>METILKMGLQANVGSVEYDSAKILSDKISELSDGEMKLLLYPGAQLGDDRAMLQQLSMGDLDITFAEFGRMGLWIPRAEAVMLPYVVKNYAHIQRIFNSKFGQGVREEMLTNFNWRALDTWYNGTRQTSSNRPLNTISDFEGLKLRVPNAKANLAFAKYAGASPTPMVFSEVYLALQTNAVDGQENPLPTFNTMKFYEVQPNLAMTNHIVNDQMVLISEDRWQSLSKDQQATITEAVSVAGKRHTNFVNNQEKELITFFKAEGVNITYPDLAPFREAMLPIYKDFDKKIGKQLVEELSDI[2x]

Tripartite ATP-independent periplasmic (TRAP) transporters are a major class of secondary transporters found in bacteria and archaea—but, not in eukaryotes. First reported over 25 years ago6, they use energetically favourable cation gradients to drive the import of specific carboxylate- and sulfonate-containing nutrients against their concentration-gradient, including C4-dicarboxylates, α-keto acids, aromatic substrates and amino acids. A functional TRAP system is made up of a soluble substrate-binding ‘P-subunit’, and a membrane-bound complex comprising a small ‘Q-subunit’ and a large ‘M-subunit’. The best characterised TRAP transporters are those for sialic acid, otherwise known as the SiaPQM system.

We determined the crystal structure of SiaP bound to Neu5Ac in a closed state at 1.04 Å resolution, as a crystal structure of substrate-loaded SiaP enables us to model the SiaPQM complex. We confirmed that SiaP binds sialic acid with nanomolar affinity and that the crystal structure is representative of the protein structure in solution. The docked structure shows two calliper-like helices of SiaP, α2 at the N-terminal lobe and α5 at the C-terminal lobe of SiaP, interact with the scaffold portion of the M-subunit. Residues R49 and N148 (SiaP) form a latch between the lobes of SiaP at the surface of the substrate binding cleft, enclosing a number of ordered solvent molecules that extend toward the substrate. One hotspot involves the invariant D181 of SiaP immediately prior to β8 and K232 on the loop between TM7 and TM8 (L7-8) of the M-subunit (right). Adjacent to this interaction, the surface-accessible, conserved K143 on the β6 strand of SiaP interacts with D36 on the loop between TM1 and TM2 of the Q-subunit (right). This strand in SiaP extends from the protein surface to the Neu5Ac binding site, with K143 located two residues upstream of the conserved R145 which directly coordinates Neu5Ac. Thus, SiaP binding to SiaQM may pull on this strand to release the substrate. Analysis of these hotspots using mutagenesis showed that K143E caused a significant reduction in transport activity (but not the ability of SiaP to bind sialic acid), though the putative interactors D36A (SiaQ) and K232A (SiaM) did not reduce transport compared to the wildtype.> GSHMSQVEKDNTQALIPTMNMARQLSEASAWELFAAQNLTSADNEKMWQAQGRMLTAQSLKINALLQALREQGFDTTAIEQQEQEISRSLRQQGELVGQRLQLRQQQQQLSQQIVAAADEIARLAQGQANNATTSAGATQAGIYDLIEQDQRQAAESALDRLIDIDLEYVNQMNELRLSALRVQQMVMNLGLEQIQKNAPTLEKQLNNAVKILQRRQIRIEDPGVRAQVATTLTTVSQYSDLLALYQQDSEISNHLQTLAQNNIAQFAQFSSEVSQLVDTIELRNQHGL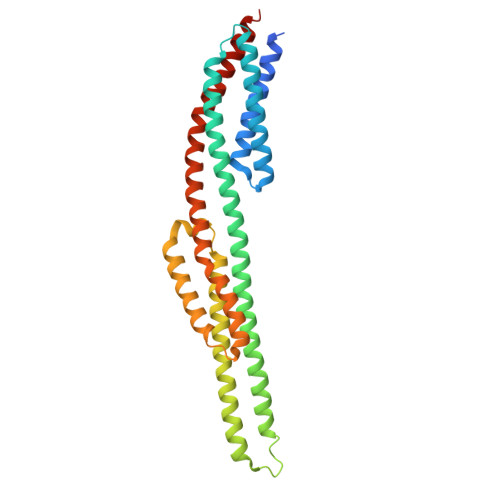A>SDVLHPYRDLFPQIGQRVMIDDSSVVIGDVRLADDVGIWPLVVIRGDVHYVQIGARTNIQDGSMLHVTHKSSYNPDGNPLTI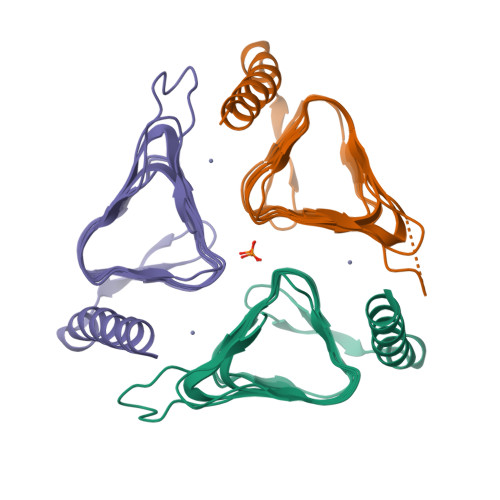GEDVTVGHKVMLHGCTIGNRVLVGMGSILLDGAIVEDDVMIGAGSLVPQNKRLESGYLYLGSPVKQIRPLSDEEKAGLRYSANNYVKWKDEYLDQGNQTQP[6x]N-{5-[(1R)-1-hydroxyethyl]-1,3-thiazol-2-yl}-alpha-D-mannopyranosylamine 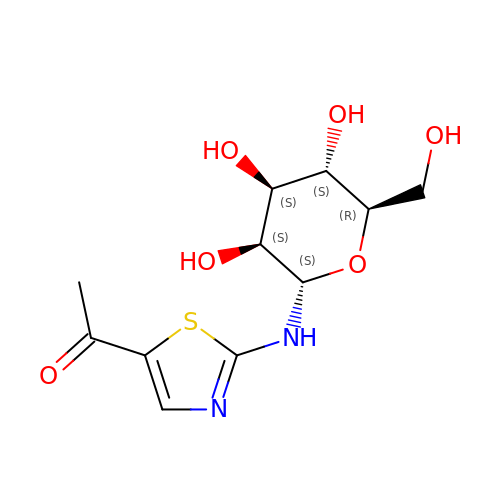| C11 H16 N2 O6 S | VVRCICGIWCXPFT-ZMLRDBKSSA-N>GPSSPSQRREHM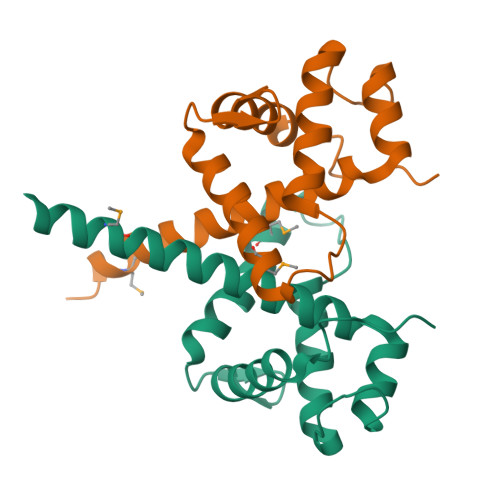LKLEAEKKKLRTILQVQYVLQNLTQEHVQKDFKGGLNGAVYLPSKELDYLIKFSKLTCPERNESLSVEDQMEQSSLYFWDLLEGSEKAVVGTTYKHLKDLLSKLLNSGYFESIPVPKNAKEKEVP[2x]BIS{[(2R,3S,4R,5R)-5-(6-AMINO-9H-PURIN-9-YL)-3,4-DIHYDROXYTETRAHYDROFURAN-2-YL]METHYL} DIHYDROGEN DIPHOSPHATE | C20 H26 N10 O13 P2 | 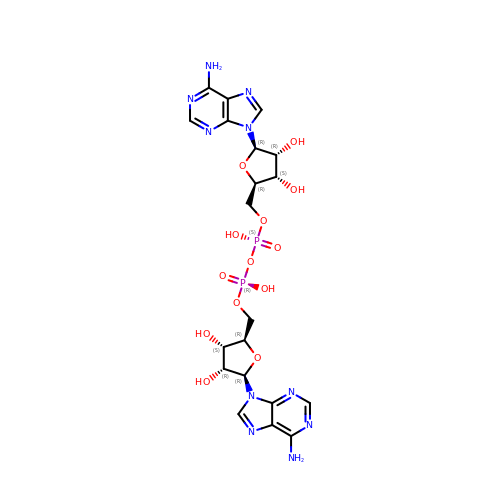AKDJDUXNKGWGAZ-XPWFQUROSA-N Proliferation and transmission of these obligate endoparasites in their host organisms rely on efficient cell invasion. This active process is based on the motility of the parasite, referred to as gliding, and is empowered by an actin/myosin motor. Actin polymerization occurs between the plasma membrane (PM) and the inner membrane complex (IMC) whereas myosin A is part of the glideosome, which binds the essential light chains ELC and myosin light chain MLC1 (called myosin tail interacting protein, MTIP, in Plasmodium spp.). MLC1 (in P. falciparum: myosin A tail-interacting protein, MTIP) binds at the very C-terminus of MyoA, while ELC is expected to interact with the C-terminus of MyoA upstream of MLC115. We demonstrate that ELCs bind to a conserved binding site on MyoA to induce its α-helical secondary structure and stiffen the MyoA neck.

To investigate whether the homologous complexes from T. gondii and P. falciparum are structurally similar, we determined the crystal structure of the P. falciparum trimeric complex (PfMyoA, MTIP, PfELC) at 2.5 Å resolution. Overall, this structure resembles a similar fold and conformation compared to the T. gondii trimeric complexes, with the typical MyoA helix kink of 131° between the MTIP and PfELC binding sites. While the secondary structure elements are maintained, the position of the PfELC helices differ. The N-terminal lobe of PfELC aligns well to TgELCs structures (backbone RMSD of 2.5 Å to TgELC1), but the C-terminal lobe adopts a different orientation with respect to the MyoA helix (backbone RMSD of 3.5 Å to TgELC1), resulting in a reduced number of polar interactions between PfELC and PfMyoA. This explains the lower binding affinity of trimeric complex formation in P. falciparum. Of note, the electron density of the PfELC C-terminal lobe is less well defined compared to the remaining structure, which is likely caused by increased flexibility of the C-terminal loop of PfELC. This is also reflected in the comparison of the calculated scattering data from the P. falciparum complex structure and the recorded SAXS data with Χ2 = 3.9. S127 does not directly interact with PfMyoA, but forms a polar interaction with PfELC residue N75, maintaining the tertiary structure of the C-terminal lobe. Contrary to T. gondii TgELCs, the homologous EF hand loop of PfELC (in isolation or in complex) is bent to the other side and does not possess the residues needed for coordination of calcium.

>SMASDMEEKFREAFILFSSCSDHIEMYKFFELMNSFGIILTNDEKAALPNDINMDYWLNFAKKHYNYEQPFKHINNVNEQNTNVQIKIDNFLGIMKALDTRLTESDLNILLQITNPENKSTLNLKTVSQKLTESI[5x];>[5x]SMESVADIQQLEEKVDESDVRIYFNEKSSGGKISIDNASYNARKLGLAPSSIDEKKIKELYGDNLTYEQYLEYLSICVHDKDNVEELIKMFAHFDNNCTGYLTKSQMKNILTTWGDALTDQEAIDALNAFSSEDNIDYKLFCEDILQ;>SVEWENCVSVIEAAILKHKYKQKVNKNIPSLLRVQAHIRKKMV[5x]> TEEQKQEIREAFDLFDADGTGTIDVKELKVAMRALGFEPKKEEIKKMISEIDKEGTGKMNFGDFLTVMTQKMSEKDTKEEILKAFKLFDDDETGKISFKNLKRVAKELGENLTDEELQEMIDEADRDGDG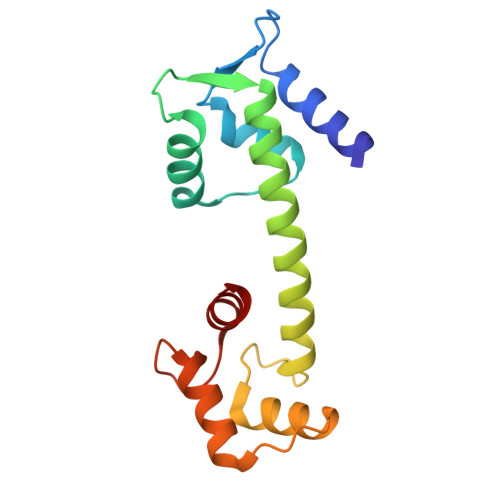EVSEQEFLRIMKK> MHHHHHHSSGRENLYFQGMGQQESTLGGAAGEPRSRGHAAGTSGGPGDHLHATPGMFVQHSTAIFSDRYKGQRVLGKGSFGEVILCKDKITGQECAVKVISKRQVKQKTDKESLLREVQLLKQLDHPNIMKLYEFFEDKGYFYLVGEVYTGGELFDEIISRKRFSEVDAARIIRQVLSGITYMHKNKIVHRDLKPENLLLESKSKDANIRIIDFGLSTHFEASKKMKDKIGTAYYIAPEVLHGTYDEKCDVWSTGVILYILLSGCPPFNGANEYDILKKVEKGKYTFELPQWKKVSESAKDLIRKMLTYVPSMRISARDALDHEWIQTYTKEQISVDVPSLDNAILNIRQFQGTQKLAQAALLYMGSKLTSQDETKELTAIFHKMDKNGDGQLDRAELIEGYKELMRMKGQDASMLDASAVEHEVDQVLDAVDFDKNGYIEYSEFVTVAMDRKTLLSRERLERAFRMFDSDNSGKISSTELATIFGVSDVDS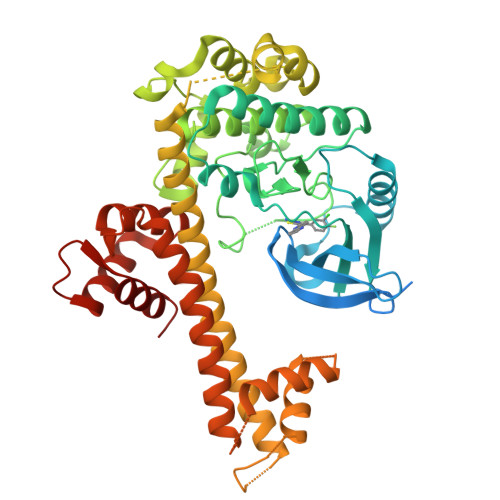ETWKSVLSEVDKNNDGEVDFDEFQQMLLKLCGN>[2x]MHEVEFSHEYWMRHALTLAKRARDEREVPVGAVLVLNNRVIGEGWNRAKGLHDPTAHAEIMALRQGGLVMQNYRLIDATLYSTFEPCVMCAGAMIHSRIGRVVFGVRNAKTHAAGSLMDVLHHPGMNHRVEITEGILADECAALLCRFFRMPRRVFNAQKKAQSSTD

To confer the favorable attributes of ABEs upon a CBE, we envisioned transforming TadA into an enzyme capable of robust cytidine deamination and subsequently generated an improved class of CBEs that uses TadA instead of a naturally occurring cytidine deaminase. Here we describe the development of two families of base editors, CABE-Ts and CBE-Ts, which use variants of TadA to catalyze the deamination of cytosines with either retention (CABE-Ts) or loss (CBE-Ts) of adenine deamination. To illuminate how amino acid substitutions identified from directed evolution affect TADAC’s substrate tolerance, we determined crystal structures of TadA*8.20 from ABE8.20-m13, the template used to evolve CABE-T1, and TADAC-1 variants from CABE-T1 reported here. Through X-ray crystallography, we show how the accumulation of substitutions impacts the shape of the active site cavity and may contribute to the accommodation of cytosine as substrate and the subsequent shift in specificity toward C-to-U deamination.

Notably, the crystal structure of TADAC-1.14 containing four substitutions (S2H, I49K, Y76I and G112H) reveals a structural difference in the loop between strands β4 and β5 (R107 to V130) on the right side of the active site cavity. This loop contains a G112H substitution that dramatically alters its flexibility and conformation relative to TadA*8.20 by introducing a bulky positively charged residue. Indeed, a comparison with the structure of TadA*8.20 bound to ssDNA substrate shows that TADAC-1.14 may engage ssDNA differently than TadA variants with strict adenine specificity. We hypothesize that residue K49 within TADAC-1.14 may contribute to the stabilization of protein–DNA interactions required for binding cytosine-containing ssDNA substrates due to its repositioning near nucleobase dC(10) (~4.5 Å).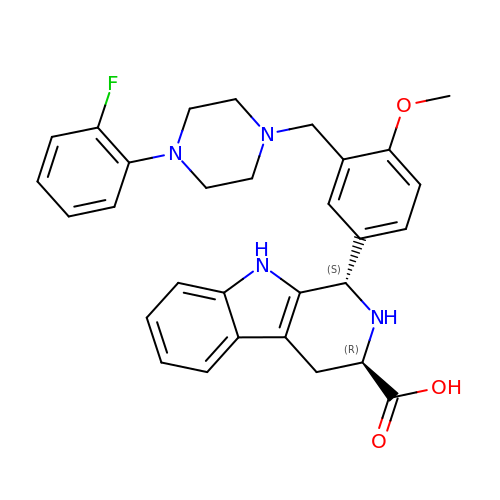(1S,3R)-1-(3-{[4-(2-fluorophenyl)piperazin-1-yl]methyl}-4-methoxyphenyl)-2,3,4,9-tetrahydro-1H-beta-carboline-3-carboxylic acid | C30 H31 F N4 O3 | FUHCEERDBRGPQZ-NAKRPHOHSA-N> KLSHVEKDFIAFYSTTPHHLSYRDKTGGSYFITRLISCFRKHACSCHLFDIFLKVQQSFEKAS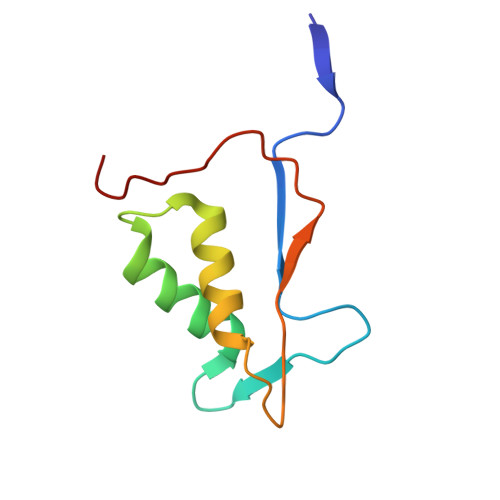IHSQMPTIDRATLTRYFYLFPGN(1R,2R,3S,4R,6S)-4,6-diamino-2,3-dihydroxycyclohexyl 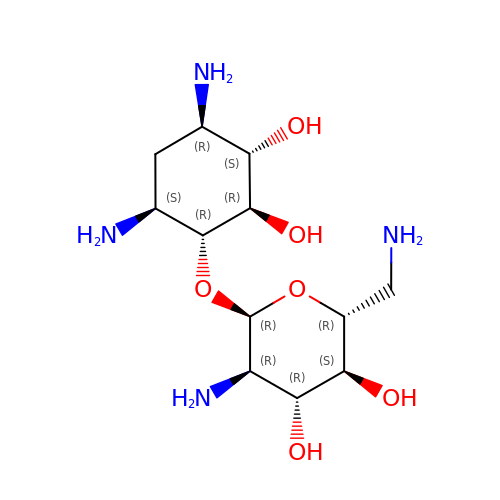2,6-diamino-2,6-dideoxy-alpha-D-glucopyranoside | C12 H26 N4 O6 | SYJXFKPQNSDJLI-HKEUSBCWSA-N1-{5-[2-(thieno[3,2-d]pyrimidin-4-ylamino)ethyl]-1,3-thiazol-2-yl}-3-[3-(trifluoromethyl)phenyl]urea | C19 H15 F3 N6 O S2 | 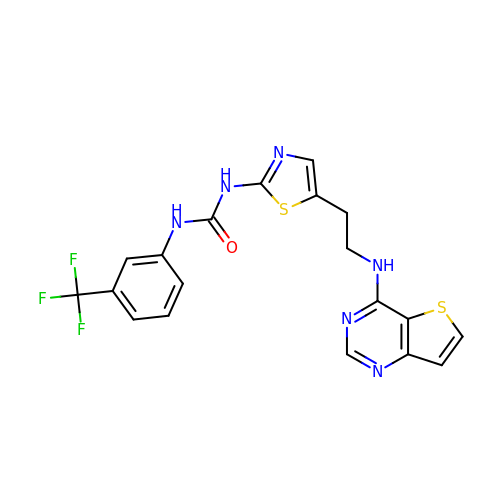JJHXPDTVQKWKHA-UHFFFAOYSA-N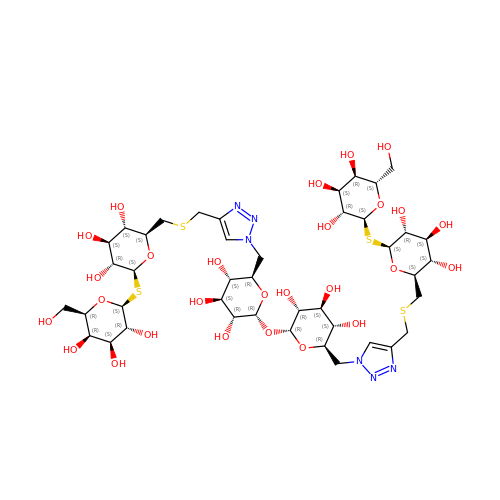(2S,3R,4S,5R,6S)-2-(hydroxymethyl)-6-{[(2S,3R,4S,5S,6S)-3,4,5-trihydroxy-6-({[(1-{[(2R,3S,4S,5R,6R)-3,4,5-trihydroxy-6-{[(2R,3R,4S,5S,6R)-3,4,5-trihydroxy-6-({4-[({[(2S,3S,4S,5R,6S)-3,4,5-trihydroxy-6-{[(2S,3R,4S,5R,6R)-3,4,5-trihydroxy-6-(hydroxymethyl)tetrahydro-2H-pyran-2-yl]sulfanyl}tetrahydro-2H-pyran-2-yl]methyl}sulfanyl)methyl]-1H-1,2,3-triazol-1-yl}methyl)tetrahydro-2H-pyran-2-yl]oxy}tetrahydro-2H-pyran-2-yl]methyl}-1H-1,2,3-triazol-4-yl)methyl]sulfanyl}methyl)tetrahydro-2H-pyran-2-yl]sulfanyl}tetrahydro-2H-pyran-3,4,5-triol | C42 H68 N6 O27 S4 | BEFBDKWEVXNDEF-GYSUOSJOSA-N> MGSDKIHHHHHHENLYFQGMQIRLAFPNEIDQIMLLIEEARAEIAKTGSDQWQKEDGYPNRNDIIDDILNGYAWVGIEDGMLATYAAVIDGHEEVYDAIYEGKWLHDNHRYLTFHRIAISNQFRGRGLAQTFLQGLIEGHKGPDFRCDTHEKNVTMQHILNKLGYQYCGKVPLDGVRL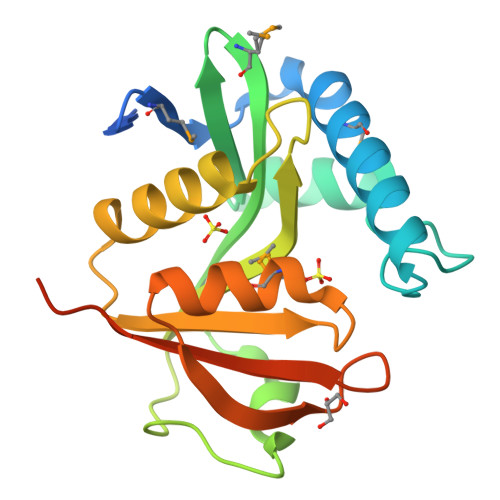AYQKIKEKGETSIYREIDERNPM> ILEAAVTQSPRNKVAVTGEKVTLSCQQTNNHNNMYWYRQDTGHGLRLIHYSYGV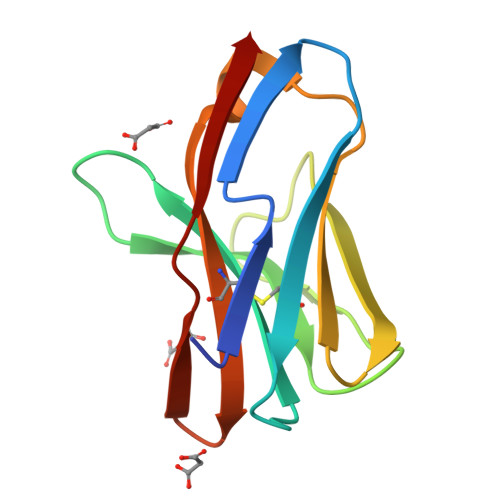GNTEKGDIPDGYKASRPSHEQFSLILVSATPSQSSVYFCASGVGGTLYFGAGTRLSVL>[2x]MNLKLQLKILSFLQFCLWGSWLTTLGSYMFVTLKFDGASIGAVYSSLGIAAVFMPALLGIVADKWLSAKWVYAICHTIGAITLFMAAQVTTPEAMFLVILINSFAYM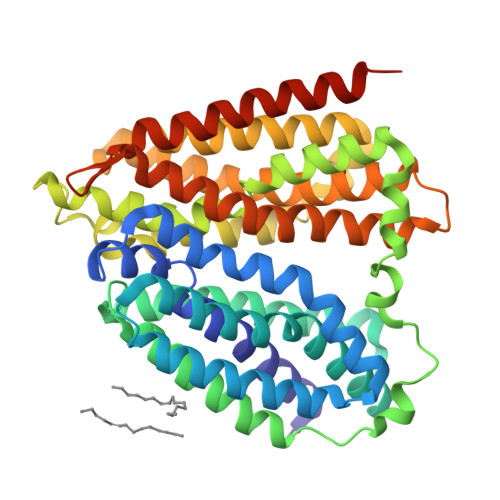PTLGLINTISYYRLQNAGMDIVTDFPPIRIWGTIGFIMAMWVVSLSGFELSHMQLYIGAALSAILVLFTLTLPHIPVAKQQANQSWTTLLGLDAFALFKNKRMAIFFIFSMLLGAELQITNMFGNTFLHSFDKDPMFASSFIVQHASIIMSISQISETLFILTIPFFLSRYGIKNVMMISIVAWILRFALFAYGDPTPFGTVLLVLSMIVYGCAFDFFNISGSVFVEKEVSPAIRASAQGMFLMMTNGFGCILGGIVSGKVVEMYTQNGITDWQTVWLIFAGYSVVLAFAFMAMFKYKHVRVPTGTQTVSH>MEASPASGPRHLMDPHIFTSNFNNGIGRHKTYLCYEVERLDNGTSVKMDQHRGFLHNQAKNLLCGFYGRHAELRFLDLVPSLQLDPAQIYRVTWFISWSPCFSWGCAGEVRAFLQENTHVRLRIFAARIYDYDPLYKEALQMLRDAGAQVSIMTYDEFKHCWDTFVDHQGCPFQPWDGLDEHSQALSGRLRAILQNQGN[2x]

The APOBEC3 family of enzymes (A3A-A3H) forms part of the innate immune response against viruses and transposons. The normally antiviral enzyme APOBEC3A is an endogenous mutagen in human cancer. Its single-stranded DNA C-to-U editing activity results in multiple mutagenic outcomes including signature single-base substitution mutations (isolated and clustered), DNA breakage, and larger-scale chromosomal aberrations. Here, we use X-ray crystallography to determine high-resolution structures of wildtype A3A/hairpin-inhibited complexes and demonstrate the underlying mechanism of inhibition.

Here we reveal the structural basis of competitive inhibition of wildtype APOBEC3A by hairpin DNA bearing 2′-deoxy-5-fluorozebularine in place of the cytidine in the TC substrate motif that is part of a 3-nucleotide loop. The hydroxyl group at C4 is coordinated to the Zn2+ center and is derived from the water/hydroxide ion bound to the Zn2+ in the substrate-free state. Tetrahedral coordination at the Zn2+ is completed by His70, Cys101, and Cys106. The catalytic glutamic acid residue, Glu72, which functions as a general acid/base, hydrogen bonds to C4-OH and N3-H of hydrated FdZ. The 5-fluoro group of FdZ is accommodated comfortably, abutting Tyr130. These results with wildtype A3A, together with prior work indicating hydration of dZ and its derivatives in structures with CDA and A3G, combine to demonstrate a universal mechanism of target nucleobase engagement, deamination, and inhibition.>SNAMKPADLTNADRIALELGHAGRNAIPYLDDDRNADRPFTLNTYRPYGYTPDRPVVVVQHGVLRNGADYRDFWIPAADRHKLLIVAPTFSDEIWPGVESYNNGRAFTAAGNPRHVDGWTYALVARVLANIRAAEIADCEQVYLFGHSAGGQFVHRLMSSQPHAPFHAVTAANPGWYTLPTFEHRFPEGLDGVGLTEDHLARLLAYPMTILAGDQDIATDDPNLPSEPAALRQGPHRYARARHYYEAGQRAAAQRGLPFGWQLQVVPGIGHDGQAMSQVCASLWFDGRMPDAAELARLAGSQSA[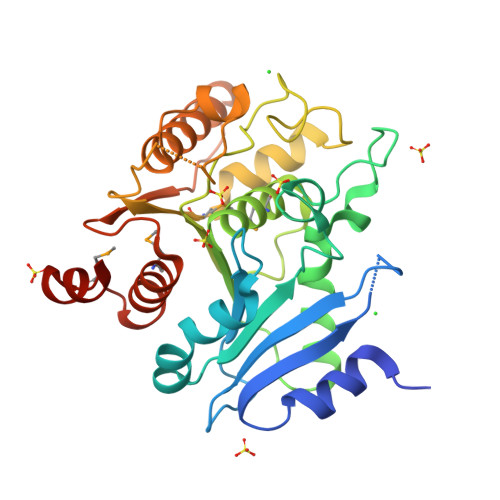2x]> ASSQLIPNISPDSFTVAASTGMLSGKSHEMLYDAETGRKISQLDWKIKNVAILKGDISWDPYSFLTLNARGWTSLASGSGNMDDYDWMNENQSEWTDHSSHPATNVNHANEYDLNVKGWLLQDENYKAGITAGYQETRFSWTATGGSYSYNN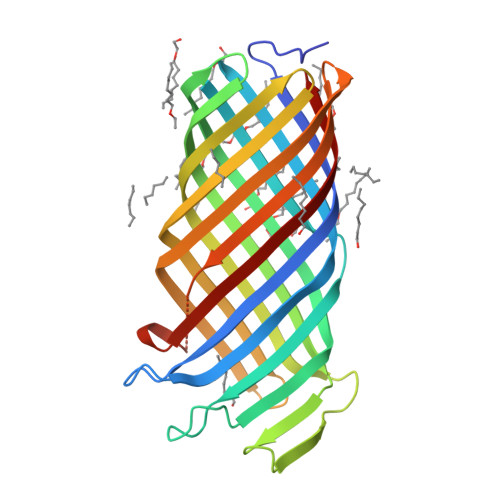GAYTGNFPKGVRVIGYNQRFSMPYIGLAGQYRINDFELNALFKFSDWVRAHDNDEHYMRDLTFREKTSGSRYYGTVINAGYYVTPNAKVFAEFTYSKYDEGKGGTQTIDKNSGDSVSIGGDAAGISNKNYTVTAGLQYRF>MHHHHHHRKAAGKYGNTLEFGHLVGGEEVLEGPLLERRNPSDREDVVARFPEADKDLVRKAALKAREAFAEWSRTPAPIRGQVLFNLVKILEREKPTLTRLMVREVGKTPKEAAGDVQEAIDTALFFASEGRRLYGQTVPSEMRDKELFTFRRPLGVVGIITAGNFPIAV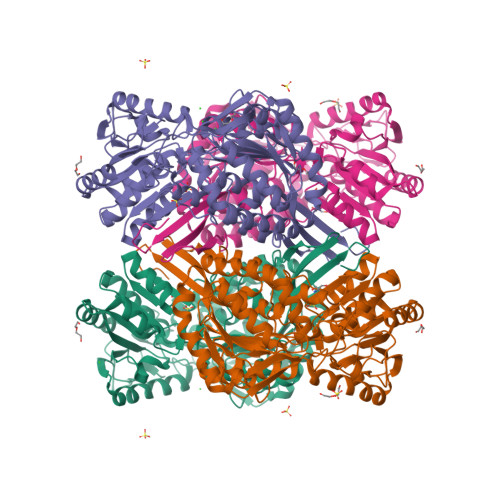PSWKLIPAVLTGNTVVWKPSEDAPTLSFVFAKLFEEAGLPPGVLNVVFGGGKGSTGQWMVELMDEGLFQKFAFTGSTQVGRWIGEVAGRNLIRPTLELGGKNPLVVMRDADLDLAVEGAWWSAFATGGQRCTSAGNILVDAPIYEEFKRRFLERVEATLVGNPLLHPEVTYGPFINERFFARWQEHYRVGEAEGARLLFGRGRITRENPYPRFLGDPEAGLYGWPTVWEVRPGTRLFTEEVFGPTINLVKVDGIEEAIAVANSTPYGLSSAIYTNHRHWAYLFKVGIRAGMTSINNATVGAEAHLPFGGVKASGNGGRESGIWVLEEYTYWHAVNEEYSGRLQLAQM[2x]>MAQTTSQVVTDIGQNAKTHTSYNTFNNEQADNMTMSLKVTFIDDPSADKQIAVINTTGSFMKANPTLSDAPVDGYPIPGASVTLRYPSQYDIAMNLQDNTSRFFHVAPTNAVEETTVTSSVSYQLGGSIDASVTPSGPSGESGATGQVDWSDSVSYDQTSYKTNLIDQTNKHVKWNVFFNGYNNQNWGIYTRDSYHALYGNQLFMYSRTYPHETDAR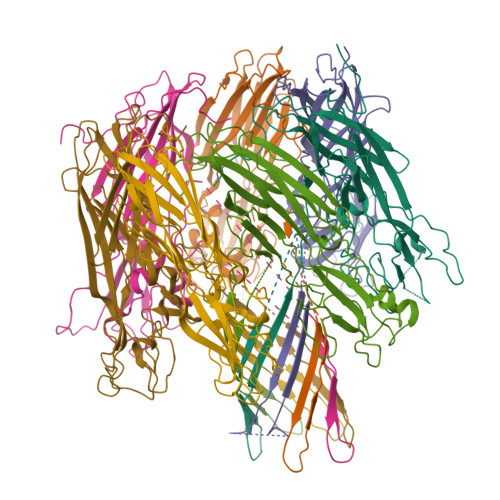GNLVPMNDLPTLTNSGFSPGMIAVVISEKDTEQSSIQVAYTKHADDYTLRPGFTFGTGNWVGNNIKDVDQKTFNKSFVLDWKNKKLVEKKGSA[7x]Non-hydrolyzing UDP-GlcNAc 2-epimerases catalyzing the reversible conversion of UDP-N-acetylglucosamine (UDP-GlcNAc) and UDP-N-acetylmannosamine (UDP-ManNAc) are central to the biosynthesis of various bacterial cell wall polysaccharides. The P. alvei MnaA enzyme (henceforth abbreviated as PaMnaA) belongs to the UDP-GlcNAc 2-epimerase protein family PF02350; structural data from 12 bacterial species are available in the Protein Data Bank (PDB). Both, monofunctional bacterial and bifunctional mammalian enzymes (vide supra) have similar folds, consisting of two Rossmann-like domains that form an active site in the cleft between them; this structure is characteristic of GT-B fold-type glycosyltransferases (GTs). Chemical evidence suggests that the catalytic mechanism of non-hydrolyzing UDP-GlcNAc 2-epimerases involves a two-step elimination-addition mechanism, with a 2-acetamidoglucal intermediate.

Crystallography on recombinant PaMnaA conducted in this study yielded an unliganded structure in 2.2-Å resolution, confirming the predicted catalytic and allosteric site of the enzyme. The crystal structure was solved at a final resolution of 2.20 Å in space group P1211 with two molecules in the asymmetric unit (AU). The PaMnaA structure contains two molecules in the crystallographic asymmetric unit, both displaying nearly identical conformations with an overlap Cα rmsd of 0.32 Å for 370 equivalent residues. As expected, the overall structure of PaMnaA forms a GT-B fold, with both the N-terminal and C-terminal domains adopting distinct Rossmann folds connected by a short linker region (residues 173–200). The space between these two folds forms an interdomain cleft containing the active site. In the absence of substrate, PaMnaA adopts an unliganded conformation corresponding to the “open” state observed for these other enzymes, where the inner surfaces of the binding cleft are exposed to solvent. This open state is believed to facilitate substrate entry and binding within the cleft. Key residues involved in substrate binding in other UDP-GlcNAc 2-epimerases are conserved in PaMnaA (R13, L18, E135, R139, H208, S285, and E291). Additionally, residues D99, E121, E135 and H208 of the putative catalytic site are conserved in the PaMnaA amino acid sequence. Overnight soaks in 10 mM UDP-α-d-GlcNAc produced no change to the resultant crystal structures, with no bound ligand observed (data not shown).

>MSKVKVMTVFGVRPEAIKMAPLILELQKHPEHIESIVCVTAQHRQMLDQVLDVFNIKPDYDLDIMQARQTLNDISVRVLQGLEPVLQEAKPDIVLVHGDTLTTFLASYAAFMQQIKVGHVEAGLRTWNKLSPFPEEMNRQLTGVLADLHFAPTDWSASNLRKENKQDASIFVTGNTVTDVFQYTVRSDYKHEVLDWAQGKRLVLMTAHRRESQGEPHRNIFRAVRRIADEFEDIAIVYPVHPSPAVREPAHEMLGDHPRIKLIDPLDVVDLHNFYPHTHLILTDSGGLQEEAPSFGIPVLVLRETTERPEGIDAGTLELVGTDEEKVYARAKALLSDETTYARMSKAANPYGDGKASQRIVSAILHSFGVLEERPEPFHTKFTNLEHHHHHH[2x]2-AMINO-4-METHYL-PENTAN-1-OL | C6 H15 N O | 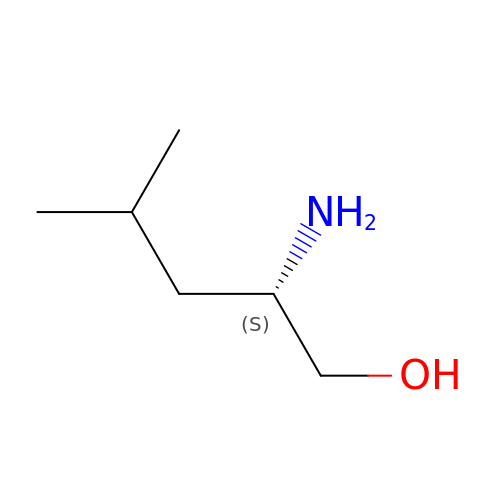VPSSPAXIFBTOHY-LURJTMIESA-N>MQDITMQWYQQLQDASMQCVLTFEGLTNSKDSQAKKIKMDLQKAATIPVSQISTIAGSKLKEIFDKIHSLLSGKPVQSGGRSVSVTLNPQGLDFVQYKLAEKFVKQGEEEVASHHEAAFPIAVVASGIWELHPRVGDLILAHLHKKCPYSVPFYPTFKEGMALEDYQRMLGYQVKDSKVEQQDNFLKRMSGMIRLYAAIIQLRWPYGNRQEIHPHGLNHGWRWLAQILNMEPLSDVTATLLFDFLEVCGNALMKQYQVQFWKMLILIKEDYFPRIEAITSSGQMGSFIRLKQFLEKCLQHKDIPVPKGFLTSSFWRS[2x];>GPSGSIIATDNVLFTPRDKLTVEELE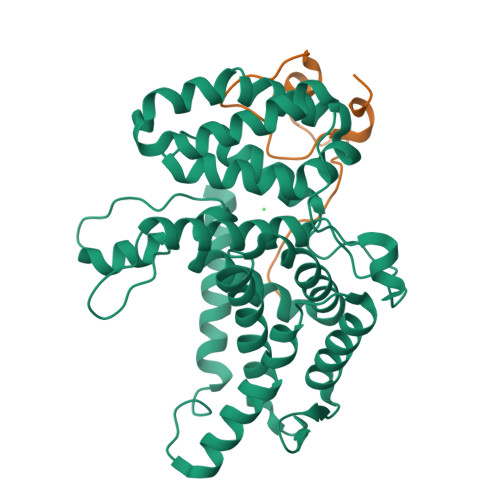QFQSKKFTLGKIPLKPPPLELLNV[2x]> GSHMAASATAAAVAAEVISVHSLEQWTMQIEEANTAKKLVVIDFTASWCGPSRIMAPVFADLAKKFPNAVFLKVDVDELKPIAEQFSVEAMPTFLFMKEGDVKDRVVGAIKEELTAKVGLHAAAQ;> MHHHHHHAADPPPVHDTDGHELRADANYYVLSANRAHGGGLTMAPGHGRHCPLFVSQDPNGQHDGFPVRITPYGVAPSDKIIRLSTDVRISFRAYTTCLQSTEWHIDSELAAGRRHVITGPVKDPSPSGRENAFRIEKYSGAEVHEYKLMSSGDWCQDLGVFRDLKGGAW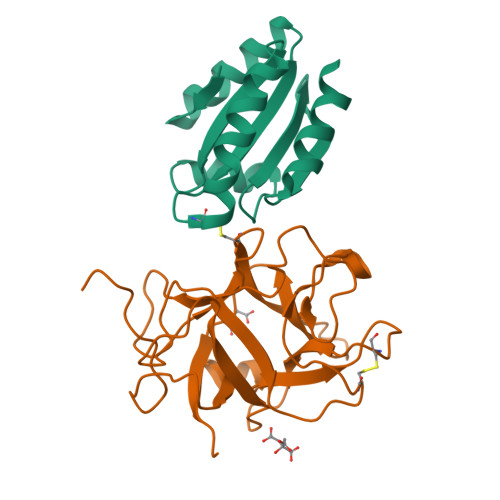FLGATEPYHVVVFKKAPPA>[2x]QLHYSVPEEAKHGTFVGRIAQDLGLELTELVPRLFRVASKDRGDLLEVNLQNGILFVNSRIDREELCGRSAECSIHLEVIVDRPLQVFHVEVEVKDINDNPPMFPATQKALFILESRL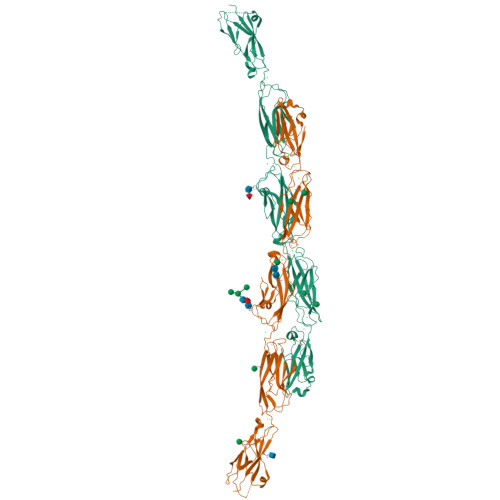LDSRFPLEGASDADVGSNALLTYRLSTNEHFSLDVPPNHEQVKPLGLVLRKPLDREEAAEIRLLLTATDGGKPELTGTVQLLITVLDVNDNAPVFDRSLYTVKLPENVPNGTLVIKVNASDLDEGVNGDVMYSFSSDVSSDIKSKFHMDTVSGEITVIGIIDFEESKAYKIPLEARDKGFPQLPGHCTILVEVVDANDNAPQLTVSSLSLPVSEDSQPGRVVTLISVFDRDSGANGQVTCSLTPHIPFKLVSTFKNYYSLVLDSALDRETIANYDVIVTARDGGSPSLWATASVSVEVADVNDNAPLFAQPEYTVFVKENNPPGAHIFTVSAMDADAQENALVSYSLVERRVGERLLSSYVSVHAESGKVFALQPLDHEELELLQFQVSARDAGVPALGSNVTLQVFVLDENDHHHHHHHH> METKTETKTGTTNFDQEALLYHQQGKPGKIEVISSKPCATEKDLSLAYSPGVAAPCKAIAKDPAKVYDYTAKGNLVAVISNGTAVLGLGNIGPAAGKPVMEGKGILFKQFAGIDVFDIEVAATDVDTFCNAVRVLEPTFGGINLEDIKAPECFEIEERLKKEMNIPVFHDDQHGTAIVSGAALLNACSITNRKMEDMRIVVNGAGASANSCAKIFIALGARRENIIMCDSQGVIYKGRTAGMNKYKEYFASETEARTLTEALRGADVFVGLSVAGALTPEMLKDMAKDPIIFAMANPEPEITPDKARAARPDAIIATGRSDYPNQVNNVLGFPSIFRGALDTRSTQINEEMKLAAVHALAKLARMDVPDKVSATYGGKSFKFGRDYLIPKPFDTRVLLWVAPEVAKAAMKSGVATRAIEDWDQYRESLEAQQGPSKVFIRSAINRVHQNSEANGGELPRIVFPEGTSTKVLKALATLVEERICQPILLGYPERVKEKIKALDIPLLNDVQIVHPSSHPKYFSFVEKLYSLRQRKGINLGEAERLMADPNYFAAMMVNMGEADGMVSGSSINYADAVRPILQTIGTYKEGIPAGLNFVLLEDKFLVLADTTVNFNPSAEQCAQIALQAAKIVEYFGIEPRVAMLSYSNFSGAEGTPRKMKKAAEIARTLRPDLMIEGDMQADTAVNPEIMERLFPFSGLKGGANVLVFPNLESSNIAYKLIQQIGKAEVIGPFLTGVRRSANVLQRTTTVDGIVNSVVFTALEAQFIKDALKARGKK

While reducing NAD(P)+ to NAD(P)H, MEs catalyze the oxidative decarboxylation of the TCA cycle intermediate L-malate to produce the TCA carbon source pyruvate and a byproduct carbon dioxide (CO2) in the presence of divalent metal ions such as a magnesium (Mg2+) ion. The hybrid-type MEs consist of an N-terminal catalytic domain (ME domain) and a C-terminal activity regulating domain. The PTA domain does not possess an enzymatic activity of PTA but acts as an allosteric modulator of catalysis; that is, binding of some metabolites to the PTA domain increases or decreases the enzymatic activity. Binding of acetyl-CoA to the PTA domain is known to reduce the catalytic activity of several hybrid-type MEs.

The cofactors NADP+ and Mg2+ were added to the protein solution prior to the data collection. First, we collected a cryo-EM data without acetyl-CoA (BbMaeBholo). In the result of 2D classification for the BbMaeBholo data, one structure with a fixed orientation of the ME domain corresponding to the H state was dominant. The structure of BbMaeBholo in the H state was determined at 2.59 Å resolution. This result is consistent with the previous crystallographic study and confirms that BbMaeB assumes the H state in the absence of acetyl-CoA.N-(3-{5-[(1,5-dimethyl-1H-pyrazol-3-yl)amino]-1-methyl-6-oxo-1,6-dihydropyridazin-3-yl}-2,6-difluorophenyl)-4,5,6,7-tetrahydro-1-benzothiophene-2-carboxamide | C25 H24 F2 N6 O2 S | 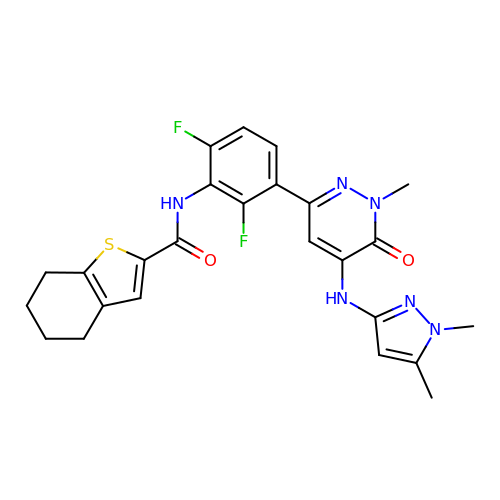CAJCMVSBNVIKHV-UHFFFAOYSA-N>GSAPSRKFFVGGNWKMNGRKQSLGELIGTLNAAKVPADTEVVCAPPTAYIDFARQKLDPKIAVAAQNCYKVTNGAFTGEISPGMIKDCGATWVVLGHSERRHVFGESDELIGQKVAHALAEGLGVIACIGEKLDEREAGITEKVVFEQTKVIADNVKDWSKVVLAYEPVWAIGTGKTATPQQAQEVHEKLRGWL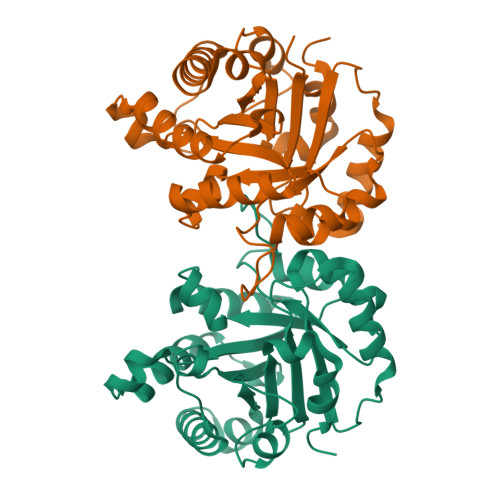KSNVSDAVAQSTRIIYGGSVTGATCKELASQPDVDGFLVGGASLKPEFVDIINAKQ[2x]>[2x]KFESKAALLAARGPEELLCFTERLEDLVCFWEEAASAGVGPGNYSFSYQLEDEPWKLCRLHQAPTARGAVRFWCSLPTADTSSFVPLELRVTAASGAPRYHRVIHINE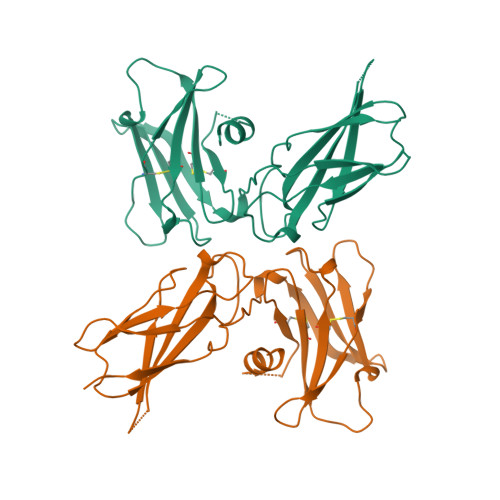VVLLDAPVGLVARLADESGHVVLRWLPPPETPMTSHIRYEVDVSAGNGAGSVQRVEILEGRTECVLSNLRGRTRYTFAVRARMAEPSFGGFWSAWSEPVSLLTPS>[2x]IVGGYTCAANSVPYQVSLNSGSHFCGGSLINSQWVVSAAHCYKSRIQVRLGEHNIDVLEGNEQFINA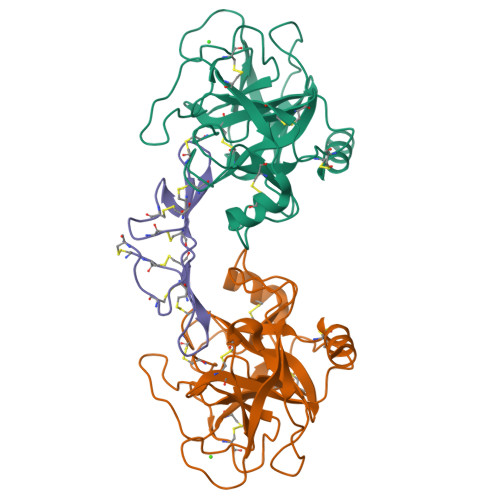AKIITHPNFNGNTLDNDIMLIKLSSPATLNSRVATVSLPRSCAAAGTECLISGWGNTKSSGSSYPSLLQCLKAPVLSDSSCKSAYPGQITGNMICVGFLEGGKDSCQGDSGGPVVCNGQLQGIVSWGYGCAQKNKPGVYTKVCNYVNWIQQTIAAN;> SHDEPSESSEPCCDSCDCTKSKPPQCHCANIRLNSCHSACKSCICTRSMPGKCRCLDTDDFCYKPCESMDKD> KSTYRTPNFDDVLKENNDADKGRSYAYFMVGAMGLLSSAGAKSTVETFISSMTATADVLAMAKVEVNLAAIPLGKNVVVKWQGKPVFIRHRTPHEIQEANSVDMSALKDPQTDADRVKDPQWLIMLGICTHLGCVPIGEAGDFGGWFCPCHGSHYDI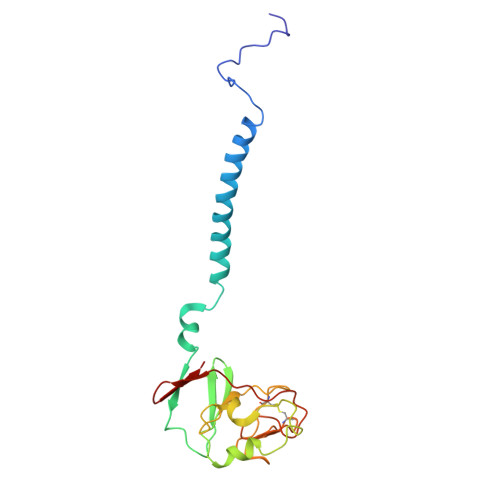SGRIRKGPAPLNLEIPAYEFDGDKVIVG>MQWSGARALEALLTVAGELRGPPLQLDTGQLLKIAKRGGVTAVEAVHAWRNALTGAPLNLTPEQVVAIASHDGGKQALETVQRLLPVLCQAHGLTPQQVVAIASHDGGKQALETVQRLLPVLCQAHGLTPEQVVAIASHDGGKQALETVQALLPVLCQAHGLTPEQVVAIASNGGGKQALETVQRLLPVLCQAHGLTPQQVVAIASNGGGKQALETVQRLLPVLCQAHGLTPQQVVAIASHAGGKQALETVQRLLPVLCQAHGLTPQQVVAIASNNGGKQALETVQRLLPVL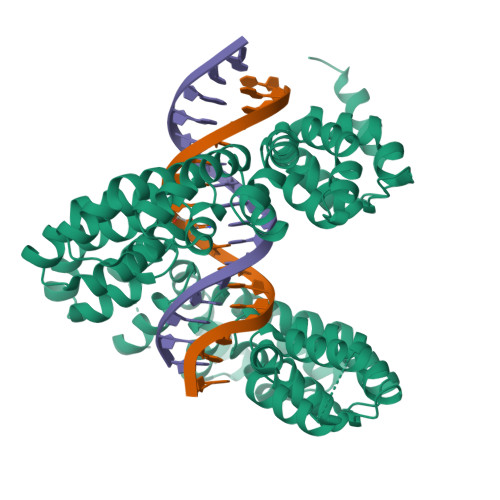CQAHGLTPQQVVAIASHDGGKQALETVQRLLPVLCQAHGLTPQQVVAIASNNGGKQALETVQRLLPVLCQAHGLTPEQVVAIASNGGGKQALETVQRLLPVLCQAHGLTPEQVVAIASHDGGKQALETVQRLLPVLCQAHGLTPQQVVAIASNGGGRPALESIVAQLSRPDPALAALTNDHLVALACLGGRPALDAVKKLEHHHHHH[2x]> MKTEWPELVGKSVE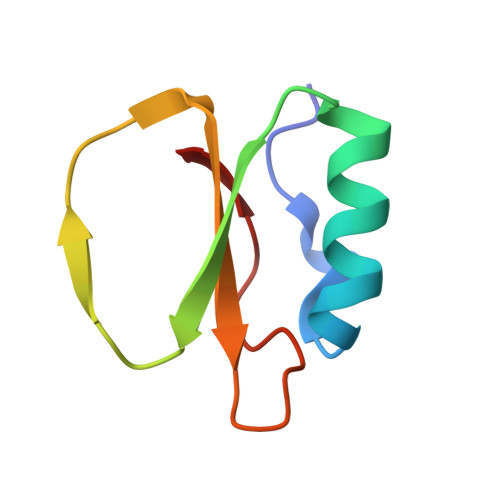EAKKVILQDKPAAQIIVLPVGTIVTMSYRIDRVRLFVDRLDNIAQVPRVG> TVFRQENVDDYYDTGEELGSGQFAVVKKCREKSTGLQYAAKFIKKRRTKSSRRGVSREDIEREVSILKEIQHPNVITLHEVYENKTDVILILELVAGGELFDFLAEKESLTEEEATEFLKQILNGVYYLHSLQIAHFDLKPENIMLLDRNVP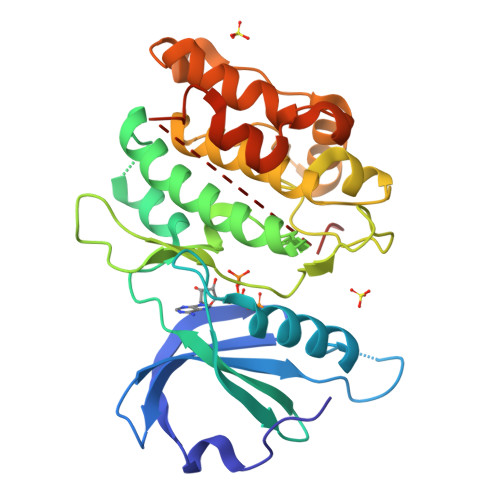KPRIKIIDFGLAHKIDFGNEFKNIFGTPEFVAPEIVNYEPLGLEADMWSIGVITYILLSGASPFLGDTKQETLANVSAVNYEFEDEYFSNTSALAKDFIRRLLVKDPKKRMTIQDSLQHPWIKPKDTQQALSSAWSHPQFEK8-Oxoguanine (GO) is a major purine oxidation product in DNA. The major way to remove GO is the base excision repair pathway, usually initiated by a GO-DNA glycosylase. While no enzymes with an A/G specific-DNA glycosylase or a dGOTPase activity have been discovered in these species, a GO-DNA glycosylase called AGOG (for Archaeal GO-DNA Glycosylase) has been initially identified in the hyperthermophilic archaeon Pyrobaculum aerophilum. Despite very low sequence identity, AGOG is structurally similar to eukaryotic and prokaryotic OGG1 and OGG2 GO-DNA glycosylases and, like these two proteins, belongs to the Endo III structural superfamily partly defined by the central helix-hairpin-helix (HhH) element followed by a glycine/proline-rich region and an aspartate (GPD).

The residues involved in GO-moiety recognition are conserved among the AGOG proteins studied so far, and we confirmed by soaking crystals in crystallization buffer containing 8-oxoguanosine (8-oxodG, Pab-AGOG + 8-oxodG) that the Pab-AGOG binding pocket has the same conformation as the one previously observed for Pae-AGOG. The damaged base is sandwiched between two aromatic residues (F146 and W212) and makes H-bonds with six Pab-AGOG residues (Q24, W62, K149, P172, D174, D208). The sugar moiety of 8-oxodG interacts through its O3’ with the carbonyl group of S51 while the O5’ establishes an intra-residual H-bond with the N2 atom of the base. Unlike Pae-AGOG, Pab-AGOG shows a change of backbone conformation at the catalytic K142 residue upon GO binding. The torsional angle Ψ of K142 has a value of 128.8° in the apo structure and of –42.9° when complexed to GO, leading to a substantial conformational change of the HhH hairpin. This conformational change could be induced and/or stabilized by the presence in the protein active site of sodium citrate coming from the crystallization buffer.

>GSHMIARIIGEIGIEGARFIEENIDEQFKALRYLSKGIDSETFVKLVIANSLVSYQLTGKGEQWWWEFAKYFYGRDVKSIYLAYKEFLPNSRFNRRLIPQKLSRIRRVETFLSTLTEERIEEYYGDMSSLWGSIARALGVDKESKTVVFSVKMFGYAARIVLSTFNPYPMEIPIPEDSRIVKLTKKLTNEKPRKFWMKIARESGVPPLHIDSILWPLLGGASIDSAPPELRDKLAELIKIIR[2x]> SATPLSGKAKVKS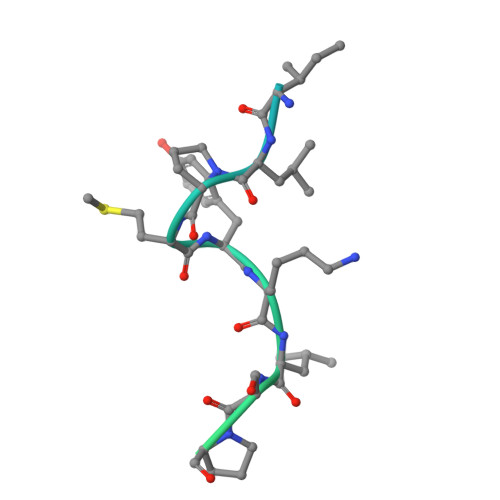RSILPMYKLSPANASRLVTTPQKRAYGFSFSAYGSPTSPSSSASSTPGAFGQSILS>GHMVTEIERKFLVATFPDGELHAVPLRQGYLTTPTDSIELRLRQQGTEYFMTLKSEGGLSRQEYEIQIDVTQFEMLWPATEGRRVEKTRYSGKLPD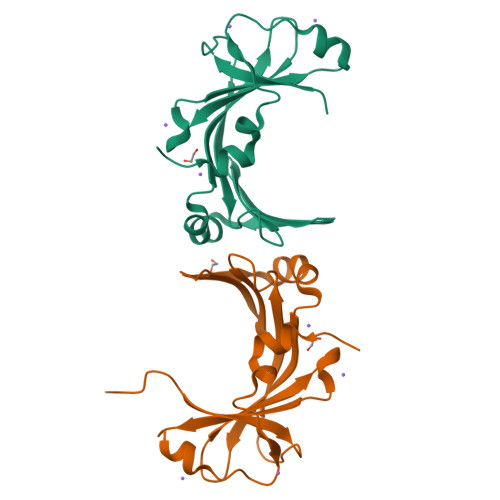GQLFELDVFAGHLSPLMLVEVEFLSEDAAQAFIPPPWFGEEVTEDKRYKNKALALSIPG[2x]> CSQSSERVVIGSKPFNEQYILANMIAILLEENGYKAEVKEGLGGTLVNYEALKRNDIQLYVEYTGTA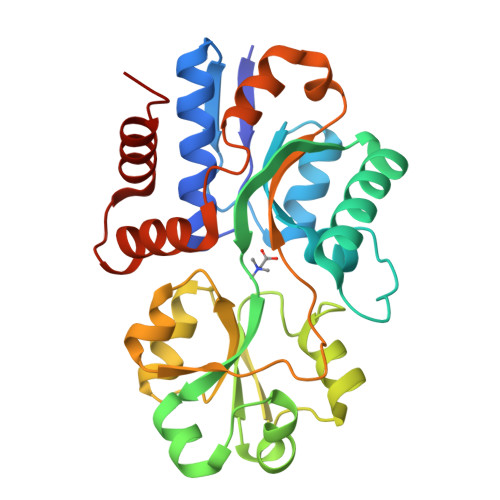YNVILRKQPPELWDQQYIFDEVKKGLLEADGVVVAAKLGFRDDYALAVRADWAEENGVEKISDLAEFADQLVFGSDPEFASRPDGLPQIKKVYGFEFKEVKQMEPTLMYEAIKNKQVDVIPAYTTDSRVDLFNLKILEDDKGALPPYDAIIIVNGNTAKDEKLISVLKLLEDRIDTDTMRALNYQYDVEKKDAREIAMSFLKEQGLVK>MGSSHHHHHHSQDPNSMTTLTRQDLNFGQV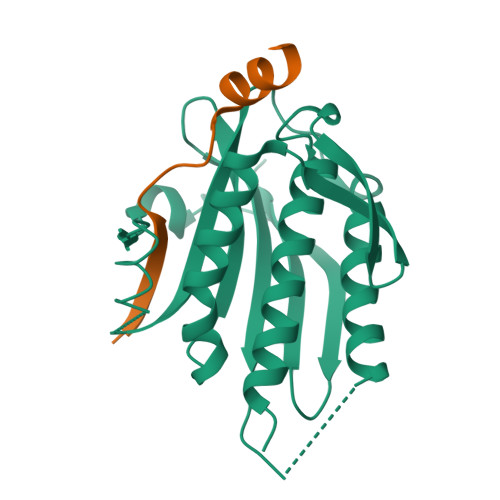VADVLCEFLEVAVHLILYVREVYPVGIFQKRKKYNVPVQMSCHPELNQYIQDTLHCVKPLLEKNDVEKVVVVILDKEHRPVEKFVFEITQPPLLSISSDSLLSHVEQLLRAFILKISVCDAVLDHNPPGCTFTVLVHTREAATRNMEKIQVIKDFPWILADEQDVHMHDPRLIPLKTMTSDILKMQLYVEERAHKGS[4x];>MEDKKIVIMPCKCAPSRQLVQVWLQAKE[4x]>[4x]MSGKLTVITGPMYSGKTTELLSFVEIY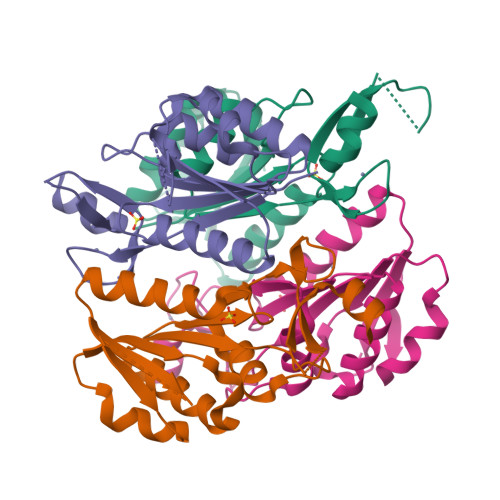KLGKKKVAVFKPKIDSRYHSTMIVSHSGNGVEAHVIERPEEMRKYIEEDTRGVFIDEVQFFNPSLFEVVKDLLDRGIDVFCAGLDLTHKQNPFETTALLLSLADTVIKKKAVCHRCGEYNATLTLKVAGGEEEIDVGGQEKYIAVCRDCYNTLKKRV>MAWNNIVFYSLGDVNSYQGGNVVITQRPQFITSWRPGIATVTWNQCNGPEFADGSWAYYREYIAWVVFPKKVMTKNGYPLFIEVHNKGSWSEENTGDNDSYFFLKGYKWDQRAFDTANLCQKPGETTRLTEKFDDIIFKVALPADLPLGDYSVTIPYTSGIQ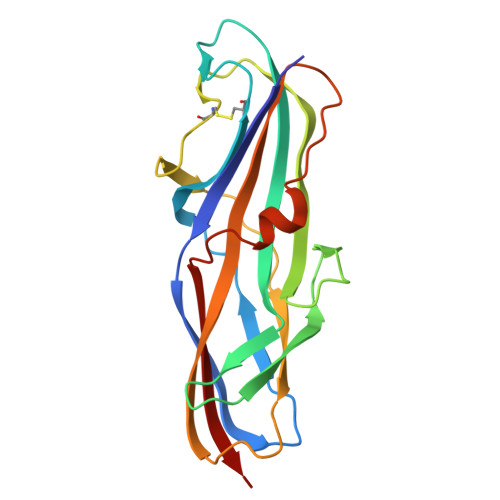RHFASYLGARFKIPYNVAKTLPRENEMLFLFKNIGG[4x]>MAHHHHHHVGTMDMAKDKGFFKKAKMEKNKRLVTPYSEECAIQIPSEIDNEQMQRMPAGGEEDQYLRIKHMSALIKKYGDLPVITTQETRLPYYWLDLFAAIDEGDTPKAHALFHLLPQDDIILRALRAVHSEDYLYQLIKYCIQAKHFGFKQLNADLVVTPKTFEILIRDCATTLFNPAKAHFSFGLPSHHAYTQMGSGFCLINKTAMLMKQAELSSAQPPKFVIIGTDVNRDNGLCDILRHSFSHLSICHIDVFDSRVYPQQDFAYINNEFNSEGVDIGKNIHVWHHNNLNYYAVDLSLTSRKSVGVHPALLFALEQLKESIREAKAKGQKIALYLPTGWDSHEDETAYCGKFVNGRMMGKTAAHQFRFNDGDLGYFYESIFTLYNENKDCVDTIYWGLEGGYDRTMYERELKILLQVIEKQLLPKDSNSHSMSY[4x]

Classical Zn2+-dependent deac(et)ylases play fundamental regulatory roles in life and are well characterized in eukaryotes regarding their structures, substrates and physiological roles. Structurally, these enzymes are composed of a central eight-stranded parallel β-sheet flanked by α-helices on each site, known as the α/β-arginase/deacetylase fold. All active site residues were conserved, as shown by the multiple sequence alignment and the structural alignment, suggesting a general acid/base catalytic mechanism for the bacterial enzymes as described for the eukaryotic counterparts. These enzymes mediate catalysis using a penta-coordinated catalytic Zn2+ ion coordinated by two aspartates and a histidine (KpHdaH (1b): Asp181, Asp269, His183).

We were able to solve two crystal structure for two Legionella enzymes of cluster 3, L. cherrii ApaH and L. pneumophila ApaH. Structurally, compared to the arginase-deacetylase core, LpApaH and LcApaH contain an additional pair of α-helices and the central parallel β-sheet is extended by a two-stranded antiparallel β-sheet. These features might be needed for recognition of the enzymes by the type IV secretion system for secretion into the host cell, or important for interaction with other proteins such as the methyltransferase RomA or the lysine acetyltransferase KAT7 in the host cells, which calls for further investigations. Notably, LcApaH and LpApaH are able to efficiently deacetylate several H3, H4, DLAT and p53-derived peptides either containing a positively charged, a negatively charged or a glycine residue at −1 position, showing a low degree of sequence specificity, which indicates that these enzymes are capable of deacylating substrates other than the previously proposed H3K14. Moreover, of all the compared enzymes, LcApaH and LpApaH were capable of removing l- and d-lactylation from lysines (Kla) in both tested peptides, the H4 peptide LGKlac and the p53-peptide QPKKlac. In LcApaH and LpApaH the XGGY-motif is conserved (LcApaH: 388-EGGY−391/LpApaH: 391-EGGY−394). The RPP-motif is substituted by the motif 176-GLPSHH-181 (LcApaH)/176-GLPSHH-181 (LpApaH), however, with highly similar main-chain traces. The structures show an open active site entry due to absence of oligomer formation and, as a consequence, the missing in trans supply of the active site lid as observed for cluster 1 and cluster 4 enzymes. Notably, for the cluster 3 enzymes LpApaH and LcApaH we discovered the highest discrepancy in the inhibitory potency between SAHA and TSA, with TSA inhibiting the enzymes almost 80–95-fold stronger.> SPSAEECGYSDRVRSITLGNSTITTQECANVVVGYGVWPEYLKDNEATAEDQPTQPDVATCRFYTLESVQWMKNSAGWWWKLPDALSQMGLFGQNMQYHYLGRTGYTIHVQCNASKFHQGCLLVVCVPEAEMGCSNLNNTPEFSELSGGDSARMFTDTQVGESNAKKVQTAVWNAGMGVGVGNLTIFPHQWINLRTN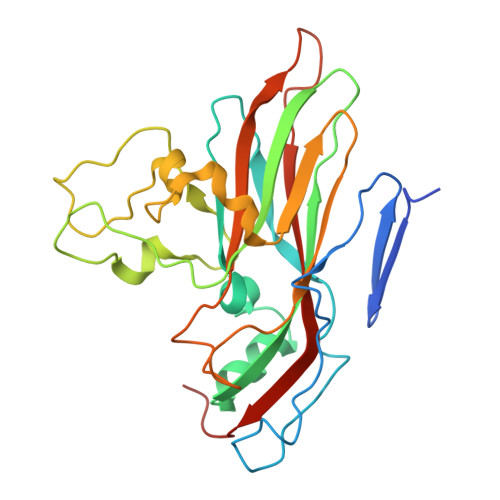NSATLVMPYINSVPMDNMFRHNNLTLMIIPFVPLNYSEGSSPYVPITVTIAPMCAEYNGLRLASNQ> MGHHHHHHHHHHSSGHENLYFQGHMANRNVEKLASIDAQLRLLVPGKVSEDDKLVEYDALLLDKFLDILQDLHGEDLKEAVQQCYELSAEYEGKHDPKKLEELGSLLTSLDTGDSIVIAKAFSHMLNLANLAEELQIAYRRRIKLKSGDFADEANATTESDIEETFKRLVHKLNKSPEEVFDALKNQTVELVLTAHPTQSVRRSLLQKHGRIRNCLAQLYAKDITPDDKQELDEALHREIQAAFRTDEIRRTPPTPQDEMRAGMSYFHETIWKGVPKFLRRVDTALKNIGINERFPYNAPLIQFSSWMGGDRDGNPRVTPEVTRDVCLLARMMTSNMYFSQIEDLMIEMSMWRCNSELRVRAEELYRTARKDVKHYIEFWKRIPPNQPYRVILGDVRDKLYNTRERSRHLLVDGKSDIPDEAVYTNVEQLLEPLELCYRSLCDCGDHVIADGSLLDFLRQVSTFGLSLVKLDIRQESDRHTEVLDAITQHLGIGSYREWSEEKRQEWLLAELSGKRPLIGPDLPKTEEVKDCLDTFKVLAELPSDCFGAYIISMATSTSDVLAVELLQREYHIKHPLRVVPLFEKLADLEAAPAAMTRLFSMDWYRNRIDGKQEVMIGYSDSGKDAGRFSAAWQLYKTQEQIVKIAKEFGVKLVIFHGRGGTVGRGGGPTHLALLSQPPDTINGSLRVTVQGEVIEQSFGEEHLCFRTLQRFCAATLEHGMNPPISPRPEWRELMDQMAVVATEEYRSVVFKEPRFVEYFRLATPELEFGRMNIGSRPSKRKPSGGI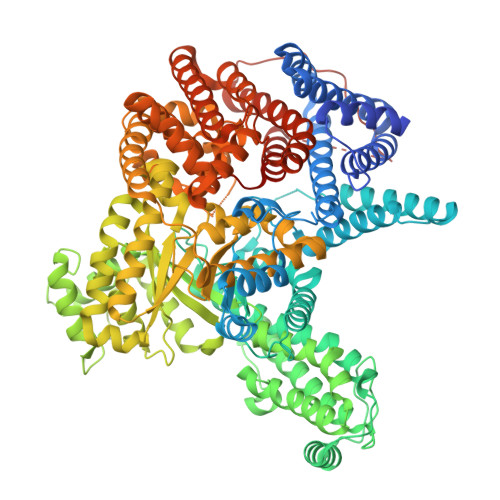ESLRAIPWIFSWTQTRFHLPVWLGFGAAFKHAIQKDSKNLQMLQEMYKTWPFFRVTIDLVEMVFAKGNPGIAALNDKLLVSEDLRPFGESLRANYEETKNYLLKIAGHKDLLEGDPYLKQGIRLRDPYITTLNVCQAYTLKRIRDPNYHVTLRPHISKEYAAEPSKPADELIHLNPTSEYAPGLEDTLILTMKGIAAGMQNTG Kinesin motor proteins hydrolyze ATP to produce force and do work in cells. Despite their diverse functions, the kinesin proteins contain a common motor domain with highly conserved or invariant sequence motifs that mediate basic motor properties, such as microtubule binding and ATP hydrolysis. For example, kinesin-14 motors move on microtubules towards the minus end instead of the plus end. Here we report a new crystal structure of human kinesin-14 KIFC1, together with new crystal structures of Drosophila Ncd, a KIFC1 orthologue, and human KIFC3, a divergent KIFC1 paralogue, and an analysis of the structural features of the proposed KIFC1 AZ82 inhibitor-binding site.

The new KIFC1 (2.25 Å) and KIFC3 (1.85 Å) structures were determined by the Structural Genomics Consortium. Both proteins were crystallized bound to Mg-ADP and are reported here for the first time. KIFC1 and KIFC3 are similar to one another in structure, but show differences in the lengths of loops, as hypothesized above. The largest difference is observed for L11, which is much shorter in KIFC3 (14 residues) than KIFC1 (30 residues), while the adjacent helix α4 is three turns longer in KIFC3 than KIFC1. Despite their relatedness, the kinesin-14 KIFC1 and KIFC3 proteins show different effects with the AZ82 inhibitor: AZ82 binds to KIFC1-MTs and inhibits both the microtubule-enhanced binding of ATP and release of nucleotide by KIFC1, but has no detectable inhibitory effects on KIFC3. In the case of the KIFC1 human homologue, KIFC3, an L5/α2/α3 pocket is visible, that again is smaller than in kinesin-5, similar to the size of the pocket in Ncd. In KIFC3, the side chain of H630, corresponding to KIFC1 R521, is not long enough to interact with L5. There are no other interactions between loop L5 and helix α3, consistent with the open conformation of the potential binding site. Kinesin-5-ADP-BI8 superposed with KIFC3-ADP shows that KIFC3 helix α4 is longer than kinesin-5 by three turns, elongating the α4/α6 pocket. Several residues of the KIFC3 α4/α6 pocket are present in similar positions as in kinesin-5, including a tyrosine, Y757, that in kinesin-5 (Y352) is thought to stack face-to-face with the benzimidazole ring of BI8.

> GSKGNIRVIARVRPVTKEDGEGPEATNAVTFDADDDSIIHLLHKGKPVSFELDKVFSPQASQQDVFQEVQALVTSCIDGFNVCIFAYGQTGAGKTYTMEGTAENPGINQRALQLLFSEVQEKASDWEYTITVSAAEIYNEVLRDLLGKEPQEKLEIRLCPDGSGQLYVPGLTEFQVQSVDDINKVFEFGHTNRTTEFTNLNEHSSRSHALLIVTVRGVDCSTGLRTTGKLNLVDLAGSERVGKSGAEGSRLREAQHINKSLSALGDVIAALRSRQGHVPFRNSKLTYLLQDSLSGDSKTLMVVQVSPVEKNTSETLYSLKFAERVRSVEL> IHTSPYSKDAPLVASLSVNQKITGRNSEKDVRHIEIDLGDSGLRYQPGDALGVWYQNDPALVKELVELLWLKGDEPVTVEGKTLPLNEALQWHFELTVNTANIVENYATLTRSETLLPLVGDKAKLQHYAATTPIVDMVRFSPAQLDAEALINLLRPLTPRLYSIASSQAEVENEVHVTVGVVRYDVEGRARAGGASSFLADRVEEEGEVRVFIEHNDNFRLPANPETPVIMIGPGTGIAPFRAFMQQRAADEAPGKNWLFFGNPHFTEDFLYQVEWQRYVKEGVLTRIDLAWSRDQKEKVYVQDKLREQGAELWRWINDGAHIYVCGDANRMAKDVEQALLEVIAEFGGMDTEAADEFLSEL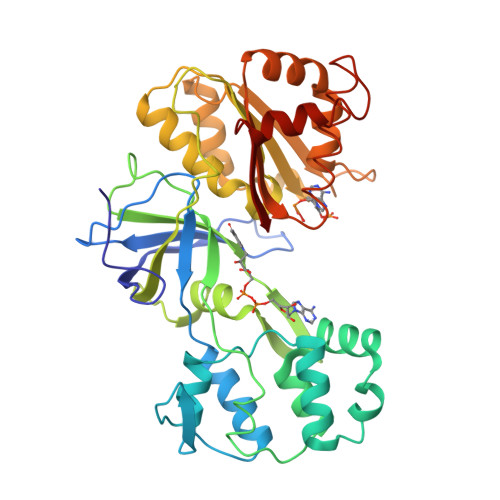RVERRYQRDVY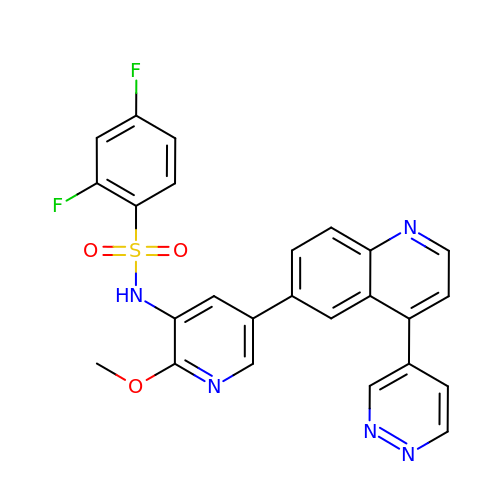2,4-difluoro-N-[2-methoxy-5-(4-pyridazin-4-ylquinolin-6-yl)pyridin-3-yl]benzenesulfonamide | C25 H17 F2 N5 O3 S | CGBJSGAELGCMKE-UHFFFAOYSA-N> MKRNYILGLDIGITSVGYGIIDYETRDVIDAGVRLFKEANVENNEGRRSKRGARRLKRRRRHRIQRVKKLLFDYNLLTDHSELSGINPYEARVKGLSQKLSEEEFSAALLHLAKRRGVHNVNEVEEDTGNELSTKEQISRNSKALEEKYVAELQLERLKKDGEVRGSINRFKTSDYVKEAKQLLKVQKAYHQLDQSFIDTYIDLLETRRTYYEGPGEGSPFGWKDIKEWYEMLMGHCTYFPEELRSVKYAYNADLYNALNDLNNLVITRDENEKLEYYEKFQIIENVFKQKKKPTLKQIAKEI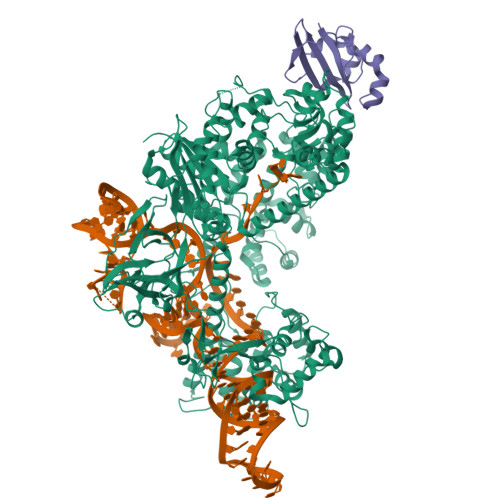LVNEEDIKGYRVTSTGKPEFTNLKVYHDIKDITARKEIIENAELLDQIAKILTIYQSSEDIQEELTNLNSELTQEEIEQISNLKGYTGTHNLSLKAINLILDELWHTNDNQIAIFNRLKLVPKKVDLSQQKEIPTTLVDDFILSPVVKRSFIQSIKVINAIIKKYGLPNDIIIELAREKNSKDAQKMINEMQKRNRQTNERIEEIIRTTGKENAKYLIEKIKLHDMQEGKCLYSLEAIPLEDLLNNPFNYEVDHIIPRSVSFDNSFNNKVLVKQEENSKKGNRTPFQYLSSSDSKISYETFKKHILNLAKGKGRISKTKKEYLLEERDINRFSVQKDFINRNLVDTRYATRGLMNLLRSYFRVNNLDVKVKSINGGFTSFLRRKWKFKKERNKGYKHHAEDALIIANADFIFKEWKKLDKAKKVMENQMFEEKQAESMPEIETEQEYKEIFITPHQIKHIKDFKDYKYSHRVDKKPNRELINDTLYSTRKDDKGNTLIVNNLNGLYDKDNDKLKKLINKSPEKLLMYHHDPQTYQKLKLIMEQYGDEKNPLYKYYEETGNYLTKYSKKDNGPVIKKIKYYGNKLNAHLDITDDYPNSRNKVVKLSLKPYRFDVYLDNGVYKFVTVKNLDVIKKENYYEVNSKCYEEAKKLKKISNQAEFIASFYNNDLIKINGELYRVIGVNNDLLNRIEVNMIDITYREYLENMNDKRPPRIIKTIASKTQSIKKYSTDILGNLYEVKSKKHPQIIKKG;> MKSVKYISNMSKQEKGYRVYVNVVNEDTDKGFLFPSVPKEVIENDKIDELFNFEHHKPYVQKAKSRYDKNGIGYKIVQLDEGFQKFIELNKEKMKENLDY Bacterial biofilm depends on the modulation of cyclic diguanylate (c-di-GMP) levels in response to environmental cues. The GGDEF domain of DGCs is emblematic of this control; since only one GTP molecule can bind in the active site, a dimerization step is mandatory for the cyclization reaction to occur and yield c-di-GMP. Consequently, multidomain DGCs usually regulate their activity by allowing the GGDEF domains to dimerize (active dimer) or forcing them apart (inactive conformations), functioning as conformational switches.

Since the dimer formation is a pre-requisite to enter DGC catalysis, we investigated the possible GMP production of the isolated GGDEF of YfiN from P. aeruginosa, an inactive truncated version, previously shown to be a monomer able to bind GTP with high affinity. According to our hypothesis, the kinetic data clearly shows that the GGDEF domain of YfiN displayed the side activity accumulating GMP, while c-di-GMP production absent. The versatile reactivity of the GGDEF domain seems to be related to a conformational issue rather than to an altered active site (as compared to the catalytically competent site required for DGC reaction): this may explain the alternative reactivity of the same protein towards GTP, depending on the allosteric status of the protein. This hypothesis has been confirmed by solving the 3D structure of the YfiNGGDEF protein in complex with Mg2+ by X-ray crystallography at 2.8 Å resolution. A magnesium ion is bound in the GTP binding site, coordinated by the oxygen atoms of D287, S288(CO), D330 (belonging to the GGDEF signature), and two water molecules. Superposition with the recently solved structure of RmcA in complex with GTP and calcium, shows that the metal ions occupy the same position and that the two water molecules replace the oxygen provided by the β and γ phosphate groups of GTP. The GTP substrate docks to the GGDEF domain in an extended conformation and a side reaction leading to the formation of c-GMP can be excluded given the position of the 3′-OH, which is too far from the α-phosphate to perform a nucleophilic attack. A closer look at the position of the phosphate groups with respect to the substrate-binding pocket indicates that the α-phosphate is particularly exposed to the solvent and, if the catalytically competent dimer does not form, may undergo a nucleophilic attack by a hydroxyl ion, thus producing GMP. For YfiN, the conserved active site, confirmed by structural data, and the high affinity for the substrate are not sufficient to promote DGC, given that the conformational activation is hampered by the upstream domain(s) truncation. Despite that the GGDEF domain is evolutionarily conserved and structurally stable, its function is strictly dependent on the neighboring domain(s) or sequences that, independently of their nature, are required to ensure the proper dimerization to enter DGC catalysis.

>GSHSWQARLQDENASLAHQAHHDSLTSLPNRAFFEGRLSRALRDANEHREQLAVLFIDSDRFKEINDRLGHAAGDTVLVNIAMRIRGQLRESDLVARLGGDEFAVLLAPLASGADALRIADNIIASMQAPIRLSDGSTVSTSLTIGIALYPEHADTPAALLHDADMAMYIAKRQARGSRRLAELNDPRILQEEKEIDSATPEAPPK[3x]> TTPLVHVASVEKGRSYEDFQKVYNAIALKLREDDEYDNYIGYGPVLVRLAWHTSGTWDKHDNTGGSYGGTYRFKKEFNDPSNAGLQNGFKFLEPIHKEFPWISSGDLFSLGGVTAVQEMQGPKIPWRCGRVDTPEDTTPDNGRLPDADKDADYVRTFFQRLNMNDREVVALMGAHALGKT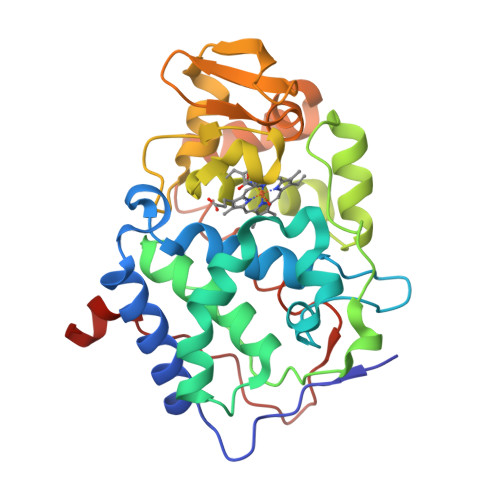HLKRSGYEGPWGAANNVFTNEFYLNLLNEDWKLEKNDANNEQWDSKSGYMMLPTBYSLIQDPKYLSIVKEYANDQDKFFKDFSKAFEKLLENGITFPKDAPSPFIFKTLEEQGL3-[6-amino-5-(3,4,5-trimethoxyphenyl)pyridin-3-yl]phenol | C20 H20 N2 O4 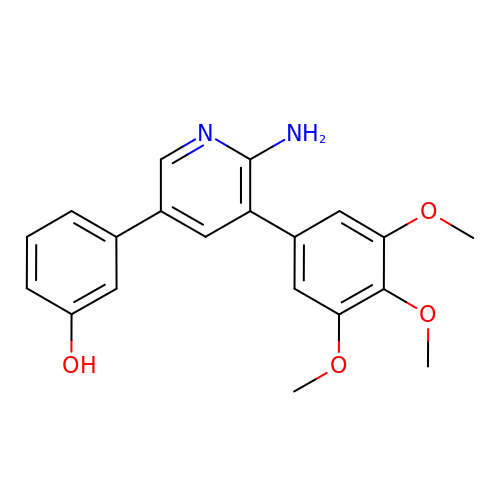| CJLMANFTWLNAKC-UHFFFAOYSA-N> MHHHHHHASDYKDDDDKGSLVPRGSPLLDDDDQVAFSFILDNIVTQKMMAVPDSWPFHHPVNKKFVPDYYKVIVNPMDLETIR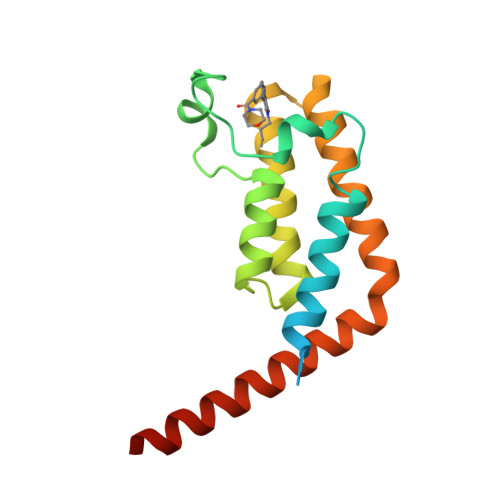KNISKHKYQSRESFLDDVNLILANSVKYNGPESQYTKTAQEIVNVCYQTLTEYDEHLTQLEKDICTAKEAALEEAELESLDPMT> GPASRPQGATVSLWETVQKWREYRRQCQRSLTEDPPPATDLFCNRTFDEYACWPDGEPGSFVNVSCPWYLPWASSVPQGHVYRFCTAEGLWLQKDNSSLPWRDLSECEESKRGERSSPEEQLLFLYIIYTVGYALSFSALVIASAILLGFRHLHCTRNYIHLNLFASFILRALSVFIKDAALKWMYSEAAQAHQWRGLLSYQDSL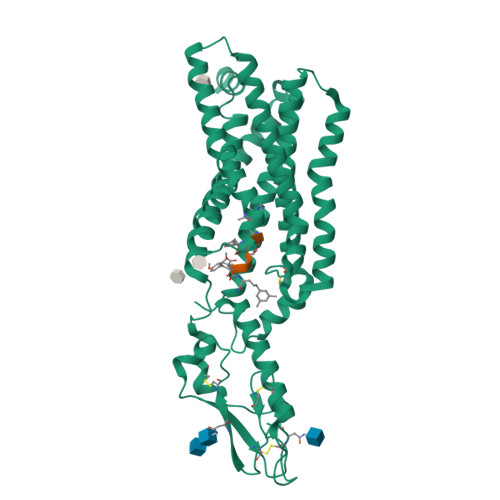SCRLVFLFMQYCVAANYYWLLVEGVYLYTLLAFSVFSEQWIFRLYVSIGWGVPLLFVVPWGIVKYLYEDEACWARNSNMNYWLIIRLPILFAIGVNFLIFVRVIAIVVSKLKANLMCKTDIKCRLAKSTLTLIALLATVEVIFAFVMDEHARGTLRFIKLFTELSFTSFQGLMVAILYCFANNEVQLEFRKSWERWRLEHLHIQRDSSAAALEVLFQ>MHHHHHHLVPRGSVHHIKRRDIVLKWELGEGAFGKVFLAECHNLLPEQDKMLVAVKALKEASESARQDFQREAELLTMLQHQHIVRFFGVCTEGRPLLMVFEYMRHGDLNRFLRSHGPDAKLLAGGEDVAPGPLGLGQLLAVASQVAAGMVYLAGLHFVHRDLATRNCLVGQGLVVKIGDFGMSRDIYSTDYYRVGGRTMLPIRWMPPESILYRKFTTESDVWSFGVVLWEIFTYGKQPWYQLSNTEAIDCITQGRELERPRACPPEVYAIMRGCWQREPQQRHSIKDVHARLQ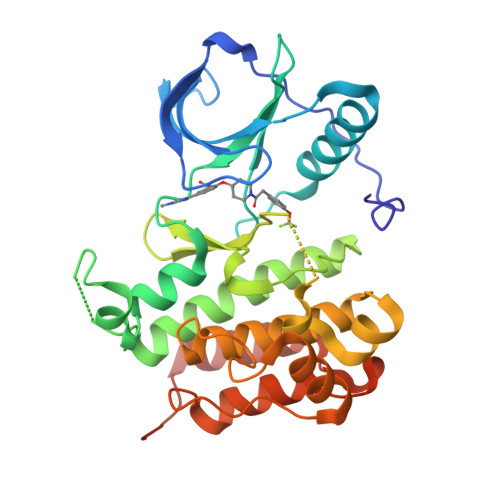ALAQAPPVYLDVLG[2x]>MAHHHHHHTDLKASSLRALKLMDLTTLNDDDTDEKVIALCHQAKTPVGNTAAIVIYPRFIPIARKTLKEQGTPEIRIATVTNFPHGNDDIDIALAETRAAIAYGADEVDVVFPYRALMAGNEQVGFDLVKACKEACAAANVLLKVIIETGELKDEALIRKASEISIKAGADFIKTSTGKVAVNATPESARIMMEVIRDMGVEKTVGFKPAAGVRTAEDAQKYLAIADELFGADWADARHYRFGASDLLASLLKALGHGDGKSASSY[2x]

Deoxyribose-5-phosphate aldolases (DERAs) are acetaldehyde-dependent, Class I aldolases catalysing in nature a reversible aldol reaction between an acetaldehyde donor (C2 compound) and glyceraldehyde-3-phosphate acceptor (C3 compound, C3P) to generate deoxyribose-5-phosphate, DRP (C5 compound). The 3D structures of several DERA enzymes have been solved, and there are also a few complex structures available. These have revealed that despite of relatively low sequence identity, all DERA enzymes have the ubiquitous TIM (α/β)8-barrel fold where the catalytic amino acids as well as other amino acid residues around the active site seem to be relatively well conserved. The DERA reaction proceeds via Schiff base formation between an active site lysine residue (K167 in Ec DERA) and the donor acetaldehyde substrate. The active site of DERA is located in a deep binding cleft, where the donor acetaldehyde binds to the bottom of the cleft and the acceptor glyceraldehyde-3-phosphate to the upper part, near the cleft entrance.

In addition, the crystal structure of one of the best Ec DERA variants, C47V/G204A/S239D, having improved activity towards acetaldehyde and basically no activity on DRP or DR, derived from the 3rd mutagenesis around, was determined from the crystal soaked with DRP. The structure of Ec DERA C47V/G204A/S239D variant was determined from crystals after soaking with DRP. The crystal structure showed a presence of a very small covalent adduct to the catalytic amino acid K167 in both molecules in the asymmetric unit. The electron density map showed elongated electron density corresponding to approximately two carbon atoms. In the refinement, it was modelled as an imine group representing a reaction intermediate. No binding of DRP or glyceraldehyde-3-phosphate could be detected. This could imply that binding of the DRP is clearly diminished in the C47V/G204A/S239D variant. The conformation of the loop containing mutation G204A has pushed the position of its Cα atom by 1.0 Å towards active site, thus narrowing it. Because the residues of this loop participate in phosphate binding (of glyceraldehyde-3-phosphate acceptor), the S239D mutation would probably decrease binding of DRP both by introducing a negatively charged amino acid residue (phosphate being also negatively charged) and by narrowing the active site entrance. On the other hand, the C47V mutation, located relatively close to the catalytic K167 residue (about 5 Å), has caused only minimal alteration in the position of this amino acid residue, as it is located in the middle of β-strand.> MTMDATALPSELLVTPQPLVGFCGLDTARVSVHKAVWEAFSGSLQRKAADRAAVQYKLLPPNYEFPVAKPKRASYEWYHPKGILKRNWMLKHLHVLPSVVVLFQDMEWNDLQWTEKQVQCAAIVQALKNTLQERNTRLCLVLLQRAAPLPPGEDLLAAERAASLTNACGITSKMLFILPHTEHLTGYALRLESAFLDMAQSYYALMSKRIRNHRDQLTAAHTSLKIRHQFKLGFVAEMRQDFSTGQKH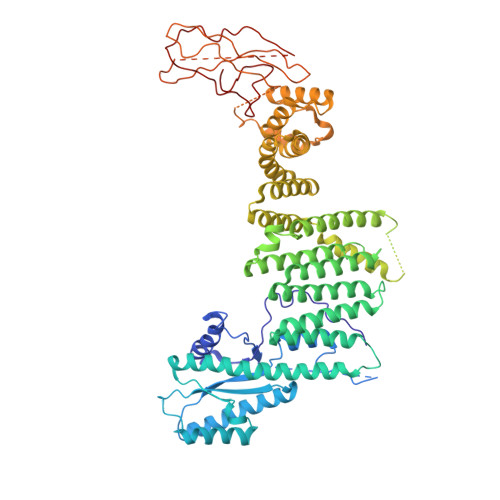YFQAYANLDEIRINDGNCLEIKTLAGFLNYKICRLMFKLKTPRDAINQFIIHVEKHKSRVGFKDLAFEHHAWLSTQHSVFAELFCEAIKNGLPALQTQHPGIYYHKAAEFVMKRRDAAMEAYAAMQASSEATPTPIQNPLSLYTEFFGIRAVKTGDLVAEQQANMQLCDQERSYNHSAAIIALLSQAMAQFKIYKCLRFRKKLAIDMAEEYLKSGDHAKALTLYSLMLPDYRQEKWTTIFTDVLLKTLRCALLSGSVADYIACSVEALSLRHQSDQSERILILENLWQVFQGVPPMPKTQLTPEAQALWTSALANVKSPIQIDLDKVNDVVEMCATFERVQLSNDDLLQLQLIVRVLTDIPLRIRSFHVILADAGNPQNSYKLEALKYFCFPTLTQLRGQKQPDDEQLENPSQEPKNFEKNMRLEPGSYYQLFCSTEAQQFHENTQLRIVRLEAHMGTDQVAALLTCSSN3-[2-bromo-4-(1H-pyrazolo[3,4-c]pyridazin-3-ylmethyl)phenoxy]-5-methylbenzonitrile | C20 H14 Br N5 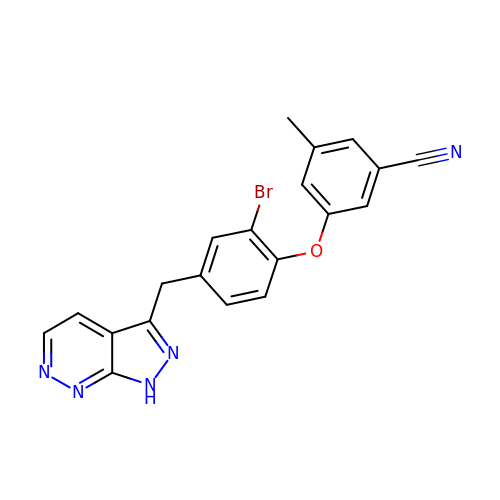O | YYGZQXRLQMFHDH-UHFFFAOYSA-N> MLNKFKLWVSKHTDYTVIHNENDLSYSIIIDFE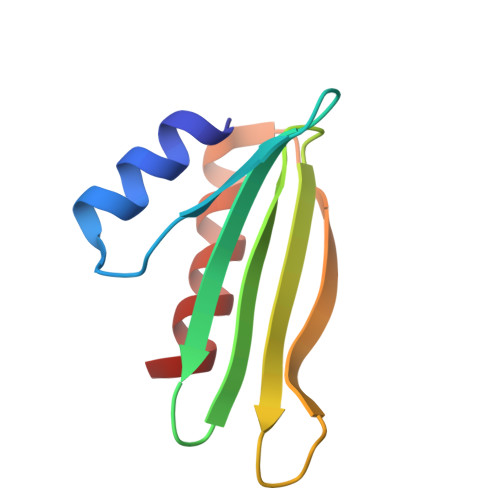DDRYISRFTVWDDLSCMSEVMDVDTGLYKLNKRNEFSTFDELLDIFDDFMISIK> MHHHHHHASENLYFQGAMGVEVCVKAAVGHPDTLGDCPFSQRVLLTLEEKKVPYEMKLIDVQNKPDWFLKISPEGKVPVFNGGDGKWIPDSDVITQVIEEKYPTPSLVTPPEYASVGSKIFSCFTTFLKSKDPNDGSEKALLTELQALEEHLKAHGPFINGQ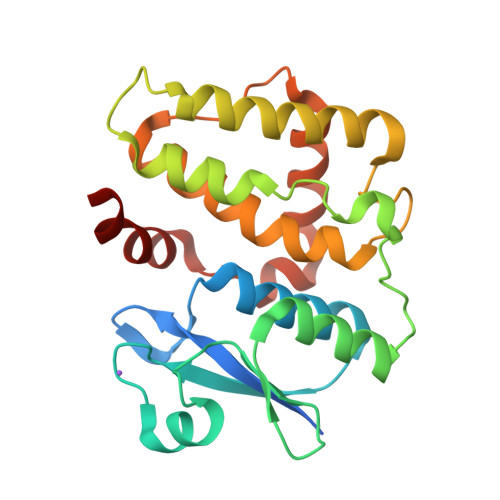NISAADLSLAPKLYHLQVALEHFKGWKIPEDLTNVHAYTEALFSRESFIKTKAAKEHLIAGWAPKVNA> EISLNGYGRFGLQYVEDRGVGLEDTIISSRLRINIVGTTETDQGVTFGAKLRMQWDDGDAFAGTAGNA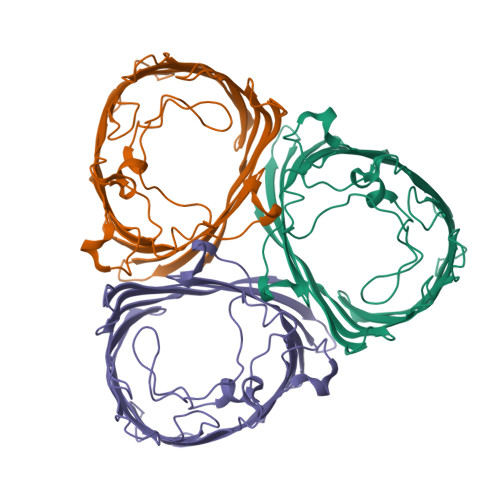AQFWTSYNGVTVSVGNVDTAFDSVALTYDSEMGYEASSFGDAQSSFFAYNSKYDASGALDNYNGIAVTYSISGVNLYLSYVDPDQTVDSSLVTEEFGIAADWSNDMISLAAAYTTDAGGIVDNDIAFVGAAYKFNGGGGPKLAKMEKARGGGGDAGTVGLNWYDNGLSTAGDQVTLYGNYAFGATTVRAYVSDIDRAGADTAYGIGADYQFAEGVKVSGSVQSGFANETVADVGVRFDF>[2x]MGSSHHHH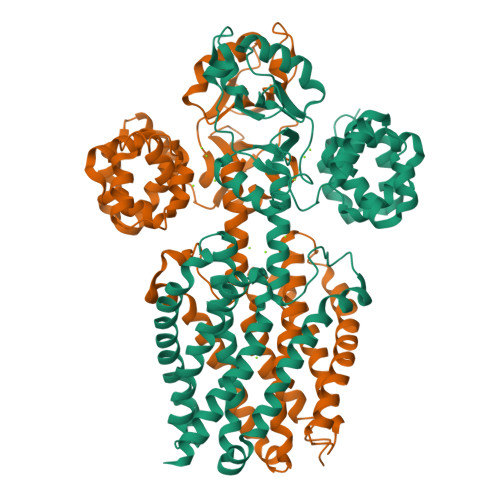HHSSGLGVLPGGPLHMEEKLAVSLQEALQEGDTRALREVLEEIHPQDLLALWDELKGEHRYVVLTLLPKAKAAEVLSHLSPEEQAEYLKTLPPWRLREILEELSLDDLADALQAVRKEDPAYFQRLKDLLDPRTRAEVEALARYEEDEAGGLMTPEYVAVREGMTVEEVLRFLRRAAPDAETIYYIYVVDEKGRLKGVLSLRDLIVADPRTRVAEIMNPKVVYVRTDTDQEEVARLMADYDFTVLPVVDEEGRLVGIVTVDDVLDVLEAEATEDIHKLGAVDVPDLVYSEAGPVALWLARVRWLVILILTGMVTSSILQGFESVLEAVTALAFYVPVLLGTGGNTGNQSATLIIRALATRDLDLRDWRRVFLKEMGVGLLLGLTLSFLLVGKVYWDGHPLLLPVVGVSLVLIVFFANLVGAMLPFLLRRLGVDPALVSNPLVATLSDVTGLLIYLSVARLLLEAV>[4x]MVISKPINARPLPAGLTASQQWTLLEWIHMAGHIETENELKAFLDQVLSQAPSE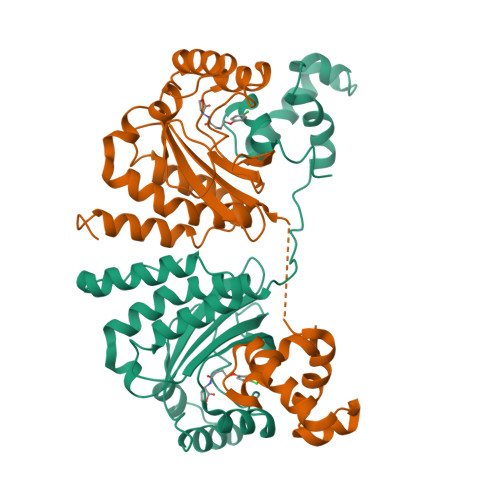RLLLALGRLNNQNQIQRLERVLNVSYPSDWLDQYMKENYAQHDPILRIHLGQGPVMWEERFNRAKGAEEKRFIAEATQNGMGSGITFSAASERNNIGSILSIAGREPGRNAALVAMLNCLTPHLHQAAIRVANLPPASPSNMPLSQREYDIFHWMSRGKTNWEIATILDISERTVKFHVANVIRKLNANNRTHAIVLGMHLAMPPSTVANE>MFNNEPLEQIDKELHDILADEEKRQRETINLIASENLTNGAVRECLGNRVSNKYSEGYPKKRYYGGNDFIDKIEELCQKRALEAFNVSDEEWGVNVQPLSGSAANVQALYALVGVKGKIMGMHLCSGGHLTHGFFDEKKKVSITSDMFESKLYKCNSQGYVDLDAVREMALSFKPKVIICGYTSYPRDIDYQQFRQICDEVNAYLFADISHISSFVACNILNNPFLHADVVTTTTHKILRGPRSALIFFNKKRNPGIEQKINSAVFPSFQGGPHNNKIAAVACQLKEVHSPAFKEYTQQVLLNSKALAKALISKQIDLVTNGTDNHLIVVDLRKFSITGSKLQETCNAINVSLNKNTIPSDVDCVSPSGVRIGTPAMTTRGAKEKDMEFIADVLARAIKITVDLQEQYGKKLVDFKKGLPGNAQLQQLKQEVVTWAGALPFP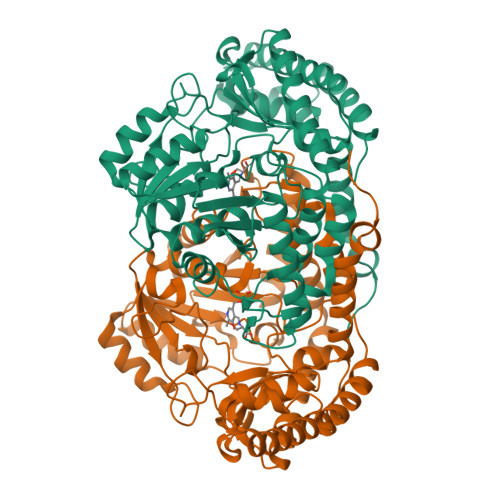[3x]>[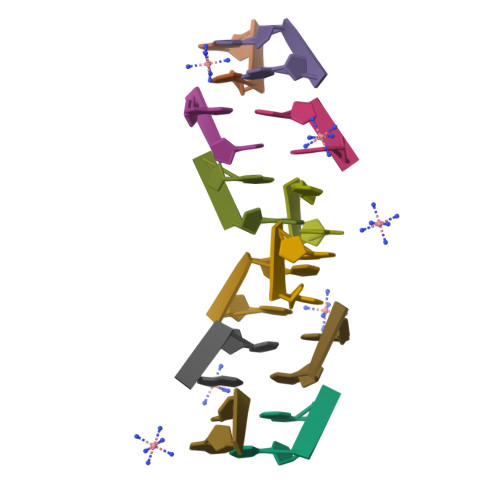2x]TG The IALB_1185 protein, which is encoded in the gene cluster for endo-β-1,2-glucanase homologs in the genome of Ignavibacterium album, is a glycoside hydrolase family (GH) 35 protein. Here, we showed using recombinant IALB_1185 that this protein has glycosyltransferase activity toward β-1,2-glucooligosaccharides, and that the kinetic parameters for β-1,2-glucooligosaccharides are not within the ranges for general GH enzymes. Kinetic analysis further revealed that the enzyme has wide aglycone specificity regardless of the anomer, and that the β-1,2-linked glucose dimer sophorose is an appropriate donor. We propose that IALB_1185 be redefined β-1,2-glucooligosaccharide:d-glucoside β-d-glucosyltransferase as a systematic name and β-1,2-glucosyltransferase as an accepted name.

In order to understand the binding modes of ligands, the complex structures of WT with glucose (Glc) and Sop2 and the complex of the E343G mutant with 1-deoxynojirimycin (DNJ) were determined. c The E343G mutant was used for the complex with DNJ. The electron densities of DNJ molecules were observed only in subunit A in the E343G mutant. The DNJ molecules are located at subsites −1 and +1 like Sop2 in the WT-Sop2 complex. The DNJ molecule at subsite +1 is well superimposed with the corresponding moiety in the WT-Sop2 complex. In contrast, the position of the other DNJ molecule shifts to a little below from the corresponding distorted Glc moiety (3H2 conformation, φ = 322.034°, θ = 125.390°, Q = 0.532, according to the Cremer–Pople parameter calculator) of the WT-Sop2 complex at subsite −1. This is probably due to pushing up of the anomeric area by the Glu343 side chain, because the potential distance between the side chain oxygen atom in the carboxy group of Glu343 and the carbon atom corresponding to an anomeric one in the DNJ molecule is too close (1.3 Å). The absence of the side chain of the residue in the E343G mutant enables accommodation of the DNJ molecule without distortion (4C1 conformation, φ = 145.774°, θ = 4.556°, Q = 0.579). The potentially too close distance between the DNJ molecule at subsite −1 and the Glu343 side chain suggests that an α-anomeric configuration of a Glc molecule is not allowed at subsite −1.

>[2x]MKPHNSEKYFVKNGQPHFLISGEVHYFRINPKLWRNHLQLLKQTGADTVSTYIPWDWHEIEEDDFDFEGKTHPARNLIRFIKLCKEENLDLIVKPGPYILAEYENQGLPSWLLKKLSKNAFALDENGNVISPDLVSYLSDEFLEYTFKWYDKVMPIISKHQKEHYGPITMMQLCNEIGVFQWLSGKSDYNPKVINLYKEFIIQRYKTIEKLNSVYSTNYNSFDDLKAPSGKIKLRSDYCAYFDFHLFFREYYNKYISILKNKIRSFGINIKLTHNIPGWIYGNASELPMLISTYSEIMKNHPDIIFGLDHIPEFVSFRNAHSDLACNKILEAMQPEAPVWAAGFQAGTREHHVKAYAKDLETFYIASLAHGIKGFNYYMFSQGINPEGKGFYGKTFYFQTALDAASNKLALYDSIKKVNRFIRKEQKDLLRTNVNSEICVGFYKPYFFTELISSQLLKEKKLNVEELGLYIDPRFLREEILFNGLLRGLQTLNYNYDVVDLENCDLKSLTAYKQLWITSAEFMDAETQNLLSEFVLNGGNLILYPAVPTLDNYLNRCEILKNNFGIEFITKDSSHKVSAFGIEDVFTAFSKKQIYNDTNSKPIAFTQENEICGIRKKIGKGELTILGFAFGYTSDEHLELIDKLVKLNKIKRELFVSDKDIQFVVRENNKSRYIFFLNYHNERKTFNYRKSSELKKKKSEEISIAPFSYKVIKENKLEHHHHHH Vinculin and its larger and muscle-specific spliced isoform called metavinculin play pivotal roles in cell adhesion by regulating cellular morphology, cellular motility, and by the transducing force between neighboring cells as well as between cells and the extracellular matrix At cell–cell and cell–matrix junctions, (meta)vinculin functions as a scaffold where it connects transmembrane cell surface receptors to the filamentous actin cytoskeleton. Vinculin and metavinculin have seven four-helix bundle domains that are connected via a about 40 residue (in vinculin) or about 100 residue (in metavinculin) flexible proline-rich linker to their respective and distinct five-helix bundle tail domains, which is called Vt in vinculin, for vinculin tail, or MVt in metavinculin, for metavinculin tail. Metavinculin has 68 amino acids inserted into the vinculin polypeptide chain between vinculin residues 915 and 916. Vinculin and metavinculin are held in their closed auto-inhibited conformers by an extensive nanomolar affinity interface between their N-terminal four-helix bundle Vh1 subdomains and their respective Vt or MVt tail domains.

To further our understanding of metavinculin activation and function, we determined the 4.17 Å cryogenic electron microscopy structure of metavinculin in its native state. The initial processing of a single ab initio three-dimensional reconstruction, including all particles accounting for best two-dimensional classes, and subsequent homogeneous refinement yielded a 4.17 Å resolution structure that overall resembled our earlier crystal structures confirming overall the auto-inhibited conformation of metavinculin. The local resolution estimate suggested that the central core is well ordered to 4.2 to 4.5 Å and contributes toward the overall resolution of the metavinculin structure. The peripheral α-helices are in the 5 to 6 Å resolution range, while a few of the surface regions exhibit resolution of less than 8 Å. While this interface is restricting the remaining domains roughly in their places, our cryogenic electron microscopy structure shows that they are surprisingly mobile. In our cryogenic electron microscopy structure, we did not observe a definitive density for the C-terminus (residues 1120 to 1134). This suggests that this region is flexible and in various conformations. The coiled coil (residues 949–960) preceding the α-helix H1’ could not be built in our cryogenic electron microscopy structures with residue 840 through 960 missing. To better resolve and visualize the molecular motions of metavinculin in detail, three-dimensional variability analyses were carried out with the default option of three modes on the entire stack of 1,303,504 particles that was subjected to homogeneous refinement. Out of the three modes computed by three-dimensional variability analyses, one mode provided a glimpse of discrete conformational states presented by metavinculin in solution.

> MPVFHTRTIESILEPVAQQISHLVIMHEEGEVDGKAIPDLTAPVAAVQAAVSNLVRVGKETVQTTEDQILKRDMPPAFIKVENACTKLVQAAQMLQSDPYSVPARDYLIDGSRGILSGTSDLLLTFDEAEVRKIIRVCKGILEYLTVAEVVETMEDLVTYTKNLGPGMTKMAKMIDERQQELTHQEHRVMLVNSMNTVKELLPVLISAMKIFVTTKNSKNQGIEEALKNRNFTVEKMSAEINEIIRVLQLTSWDEDAWASKDTEAMKRALASIDSKLNQAKGWLRDPSASPGDAGEQAIRQILDEAGKVGELCAGKERREILGTCKMLGQMTDQVADLRARGQGSSPVAMQKAQQVSQGLDVLTAKVENAARKLEAMTNSKQSIAKKIDAAQNWLADPNGGPEGEEQIRGALAEARKIAELCDDPKERDDILRSLGEISALTSKLADLRRQGKGDSPEARALAKQVATALQNLQTKTNRAVANSRPAKAAVHLEGKIEQAQRWIDNPTVDDRGVGQAAIRGLVAEGHRLANVMMGPYRQDLLAKCDRVDQLTAQLADLAARGEGESPQARALASQLQDSLKDLKARMQEAMTQEVSDVFSDTTTPIKLLAVAATAPPDAPNREEVFDERAANFENHSGKLGATAEKAAAVGTANKSTVEGIQASVKTARELTPQVVSAARILLRNPGNQAAYEHFETMKNQWIDNVEKMTGLVDEAIDTKSLLDASEEAIKKDLDKCKVAMANIQPQMLVAGATSIARRANRILLVAKREVENSEDPKFREAVKAASDELSKTISPMVMDAKAVAGNISDPGLQKSFLDSGYRILGAVAKVREAFQPQEPDFPPPPPDLEQLRLTDELAPPKPPLPEGEVPPPRPPPPEEKDEEFPEQKAGEVINQPMMMAARQLHDEARKWSSKPGIPAAEVGIGVVAEADAADAAGFPVPPDMEDDYEPELLLMPSNQPVNQPILAAAQSLHREATKWSSKGNDIIAAAKRMALLMAEMSRLVRGGSGTKRALIQCAKDIAKASDEVTRLAKEVAKQCTDKRIRTNLLQVCERIPTISTQLKILSTVKATMLGRTNISDEESEQATEMLVHNAQNLMQSVKETVREAEAASIKIRTDAGFTLRWVRKTPWYQHHHHHHHH>[3x]HHHHHHSSGLVPRGSHMSCEELEIVWNNIKAEARTLADCEPMLASFYHATLLKHENLGSALSYMLANKLSSPIMPAIAIREVVEEAYAADPEMIASAACDIQAVRTRDPAVDKYSTPLLYLKGFHAL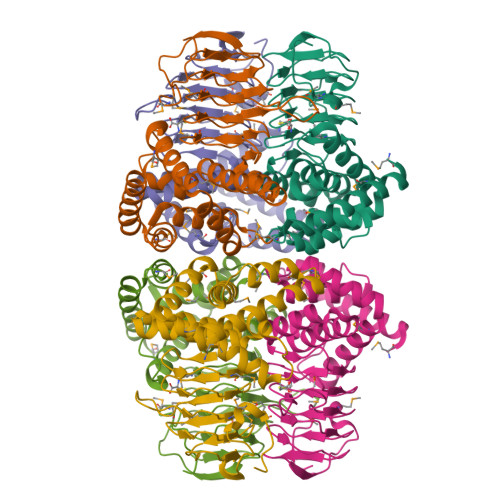QAYRIGHWLWNQGRRALAIFLQNQVSVTFQVDIHPAAKIGRGIMLDHATGIVVGETAVIENDVSILQSVTLGGTGKSGGDRHPKIREGVMIGAGAKILGNIEVGRGAKIGAGSVVLQPVPPHTTAAGVPARIVGKPDSDKPSMDMDQHFNGINHTFEYGDGI>MPAPEAPTSTLPPERPLTNLQQQIQQLVSRQPNLTAGLYFFNLDSGASLNVGGDQVFPAASTIKFPILVAFFKAVDEGRVTLQERLTMRPDLIAPEAGTLQYQKPNSQYAALEVAELMITISDNTATNMIIDRLGGAAELNQQFQEWGLENTVINNPEPDMKGTNTTSPRDLATLMLKIGQGEILSPRSRDRLLDIMRRTVTNTLLPAGLGKGATIAHKTGDIGIVVGDAGMVDMPNGQRYVAAMMVKR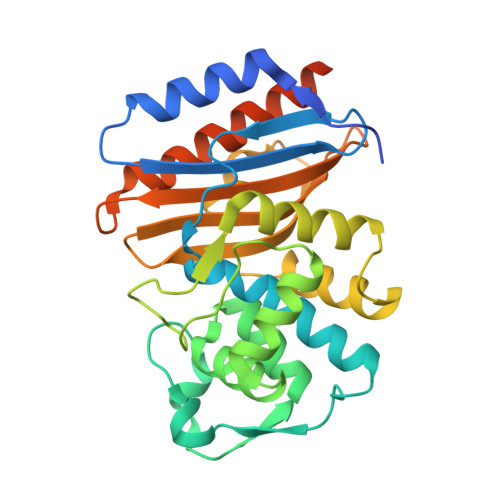PYNDPRGSELIRQVSRMVYQAFEKLSPPEQKLISEEDLNSAVDHHHHHH[4x]>[12x]SNA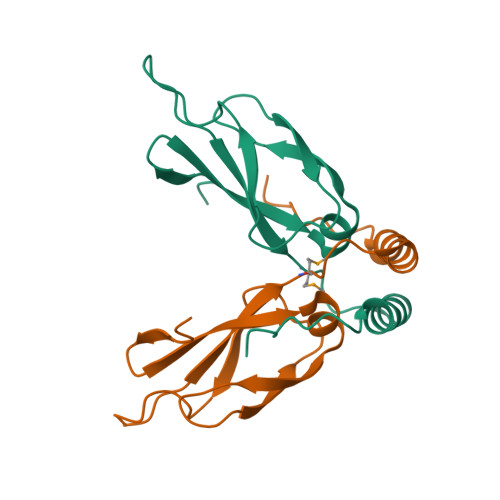HPLFDIVGHNLEIVLPLAPWEAALGAKVTVPTLKESILLTVPPGSQAGQRLRIKGKGLVSKTHTGDLFAVIKIVMPTKPDEKARELWQQLAAAEASFDPRKTWGKA> MATLKRDKGLDNTLKVLKQGYLYTTNQRNRLNTSVFQTKALGGKPFVVVTGKEGAEMFYNNDVVQREGMLPKRIVNTLFGKGAIQTVDGKKHVDRKALFMS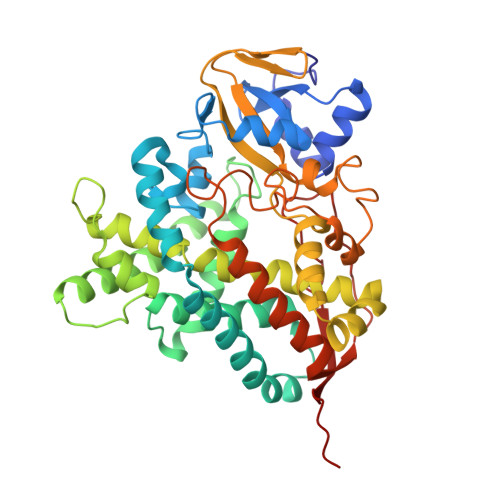LMTEGNLNYVRELTRTLWHANTQRMESMDEVNIYRESIVLLTKVGTRWAGVQAPPEDIERIATDMDIMIDSFRALGGAFKGYKASKEARRRVEDWLEEQIIETRKGNIHPPEGTALYEFAHWEDYLGNPMDSRTCAIDLMNTFRPLIAINRFVSFGLHAMNENPITREKIKSEPDYAYKFAQEVRRYYPFVPFLPGKAKVDIDFQGVTIPAGVGLALDVYGTTHDESLWDDPNEFRPERFETWDGSPFDLIPQGGGDYWTNHRCAGEWITVIIMEETMKYFAEKITYDVPEQDLEVDLNSIPGYVKSGFVIKNVREVVDRT>MRGSHHHHHHGSMVSKGEELIKENMHMKLYMEGTVNNHHFKCTSEGEGKPYEGTQTQRIKVV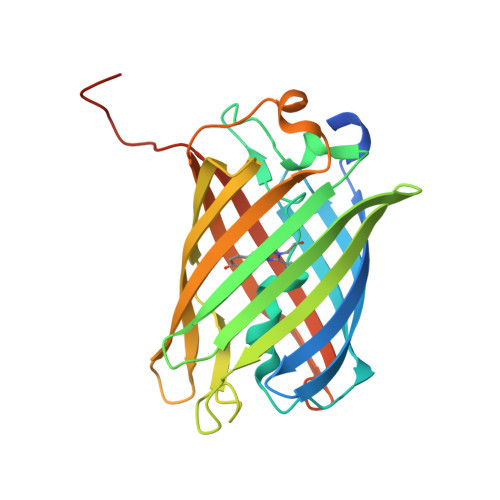EGGPLPFAFDILATCFMYGSKTFINHTQGIPDFFKQSFPEGFTWERVTTYEDGGVLTATQDTSLQDGCLIYNVKIRGVNFPSNGPVMQKKTLGWEANTETLYPADGGLRGHNPMALKLVGGGHLICNLKTTYRSKKPAKNLKMPGVYFVDRRLERIKEADNETYVEQHEVAVARYCDLPSKLGHKLNGMDELYK[4x]> SSVKRQSTARTRSFTETNR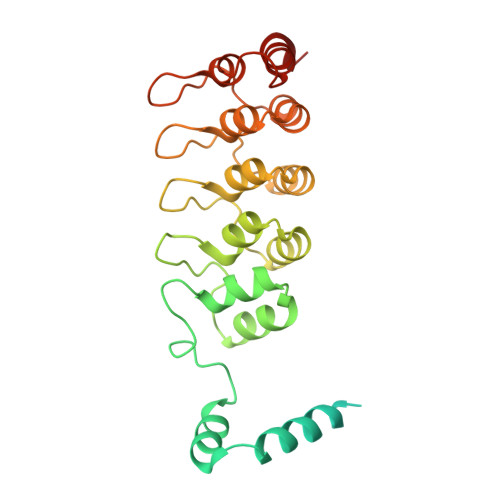RTPSVQSKHEFWEDPDDGSDSENEYEGEEEDGIGNDLDNESDWEDDSRVQKLTTTDNYEEELAKEVEQLLEPEERVILQQNEKPNLKMISTKSWKPLQTLALSMQIQLMDNLIENGLDIDDVDKDNQTALHKAIIGKKEAVISHLLRKGANPHLQDRDGAAPIHYAVQVGALQTVKLLFKYNVDVNVADNEGWTPLHIAVQSRNRDITKILLTNGADKTRRTKDGKLALDLALCFGRDFKSYDLVKLLKIMPTGDI> MHHHHHHSSGMNWTVDIPIDQLP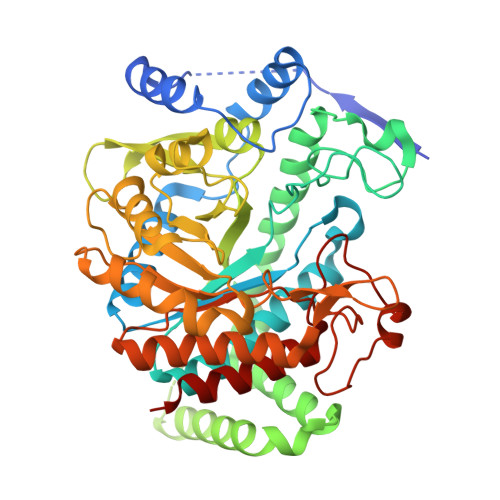SLPPLPTDLRTRLDAALAKPAAQQPTWPADQALAMRTVLESVPPVTVPSEIVRLQEQLAQVAKGEAFLLQGGDCAETFMDNTEPHIRGNVRALLQMAVVLTYGASMPVVKVARIAGQYAKPRSADIDALGLRSYRGDMINGFAPDAAAREHDPSRLVRAYANASAAMNLVRALTSSGLASLHLVHDWNREFVRTSPAGARYEALATEIDRGLRFMSACGVADRNLQTAEIYASHEALVLDYERAMLRLSDGDDGEPQLFDLSAHTVWIGERTRQIDGAHIAFAQVIANPVGVKLGPNMTPELAVEYVERLDPHNKPGRLTLVSRMGNHKVRDLLPPIVEKVQATGHQVIWQCDPMHGNTHESSTGFKTRHFDRIVDEVQGFFEVHRALGTHPGGIHVEITGENVTECLGGAQDISETDLAGRYETACDPRLNTQQSLELAFLVAEMLRD>MLQGLNHLTLAVSDLASSLAFYQQLPGMRLHASWDSGAYLSCGAL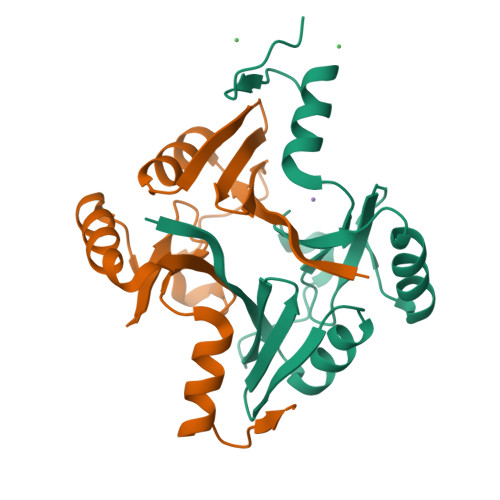WLCLSLDEQRRKTPPQESDYTHYAFSVAEEEFAGVVALLAQAGAEVWKDNRSEGASYYFLDPDGHKLELHVGNLAQRLAACRERPYKGMVFFDHHHHHH[8x]>[3x]GPTADLGAVIDFSEAHLARSPKPGVPQVVRFPLNVSSVTERDAERVGLEPVSKWRAYGLEGYPGFIFIPNPFLPGCQRHWVKQCLKLYSQKPNVCNLDKHMTKEET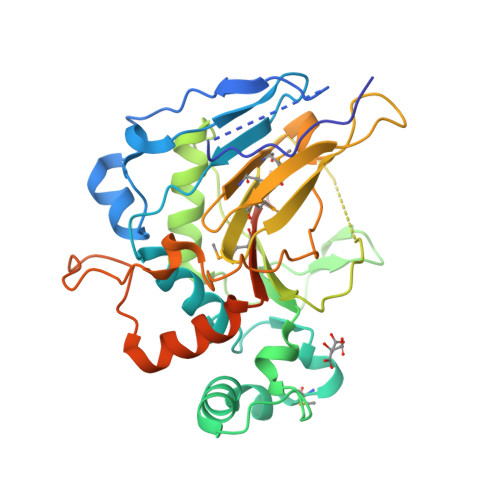QGLWEQSKEVLRSKEVTKRRPRSLLERLRWVTLGYHYNWDSKKYSADHYTPFPSDLAFLSEQVATACGFQGFQAEAGILNYYRLDSTLGIHVDRSELDHSKPLLSFSFGQSAIFLLGGLKRDEAPTAMFMHSGDIMVMSGFSRLLNHAVPRVLPHPDGECLPHCLETPLPAVLPSNSLVEPCSVEDWQVCATYLRTARVNMTVRQVLATGQDFPLEPVEETKRDIAADG>[2x]GCGUACGAAGGAGAGGAGAGGUAGAGGAGAGUACG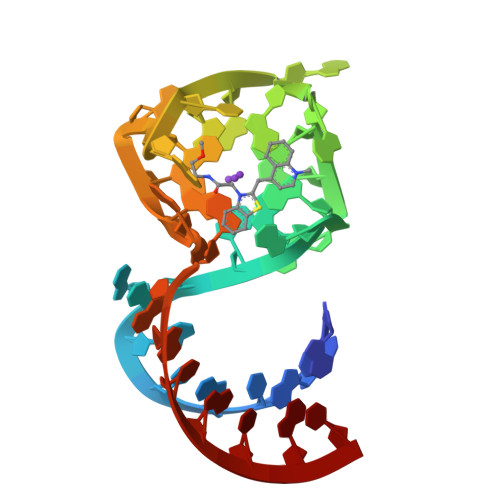C;> CGUACGAAGGAGAGGAGAGGUAGAGGAGAGUACGG>ASKWTYFGPDGENSWSKKYPSCGGLLQSPIDLHSDILQYDASLTPLEFQGYNLSANKQFLLTNNGHSVKLNLPSDMHIQGLQSRYSATQLHLHWGNPNDPHGSEHTVSGQHFAAELHIVHYNSDLYPDASTASNKSEGLAVLAVLIEMGSFNPSYDKIFSHLQHVKYKGQEAFVPGFNIEELLPERTAEYYRYRGSLTTPPCNPTVLWTVFRNPVQISQEQLLALETALYCTHMDDPSPREMINNFRQVQKFDERLVYTSFSQ[4x]

The role of carbonic anhydrase isozyme IX (CAIX) in tumor cell survival, proliferation, migration, pH regulation, and cell-signaling pathways made this enzyme a promising therapeutic target in oncology. , Tumor cells primarily express two membrane-associated carbonic anhydrases, CAIX and CAXII. These isozymes belong to a family of zinc metalloenzymes that catalyze the reversible hydration of CO2 to form HCO3 – and H+. Although the active site is characterized by conserved amino acids between 12 isozymes, the amino acids further away from the zinc ion provide some variability. Crystal structures of CAIX and CAXII with five compounds by using soaking or cocrystallization were determined to confirm the binding mode of the ligands and reveal insights that govern enhanced affinity.

Four ligands in complexes with CAXII are of similar structures, contain a cyclooctylamine group at the 3-position and (3-hydroxypropyl)­sulfonyl tail at the 4-position, but vary in substituents at the 5-position: compound 9 has a (4-hydroxybutyl)­amino moiety, compound 10 - piperidinyl, compound 13 - methoxy, and compound 14 - ethoxy. The introduction of methoxy (compound 13) and ethoxy (compound 14) groups at the 5-position of fluorinated benzenesulfonamide 5c resulted in the most strongly binding compounds for CAIX, with the K d,obs reaching 4.5 pM at pH 7.0. The elongation of the 5-substituent from methoxy to ethoxy decreased binding to CAVB by 12.8-fold and to CAXIII by 6.8-fold, whereas other anhydrases showed up to 2-fold change in affinity. Interestingly, cancer-related CAXII also interacts strongly with 13 and 14, exhibiting 0.05 nM and 0.11 nM binding affinities, respectively. Complexes of CAXII-13 and CAXII-14 each have four subunits in both duplicate structures, and the ligands adopt nearly identical conformations across all eight subunits. First, the meta cyclooctylamino group is positioned in a hydrophobic region of the active site, making the main contacts with A129-S130 (main chain), V119, S133, and side chains of L197 and L139. The meta-ethoxy group in compound 14 is oriented similarly within the hydrophilic region of the active site, but unlike compound 13, there is no space for a water molecule between the ligand and protein side chains. The hydroxyl tail is oriented against the backbone of P200–P201, forming a hydrogen bond with the main chain oxygen of P200 in most subunits. Interestingly, despite the bulkiness of synthesized di-meta-substituted compounds 10, 13, and 14, especially the first one compound 10, which possesses large piperidinyl and cyclooctylamino groups, ligands acquire quite similar binding poses in the soaked and cocrystallized complexes with CAXII.>[4x]PPYTVVYFPVRGRCAALRMLLADQGQSWKEEVVTVETWQEGSLKASCLYGQLPKFQDGDLTLYQSNTILRHLGRTLGLYGKDQQEAALVDMVNDGVED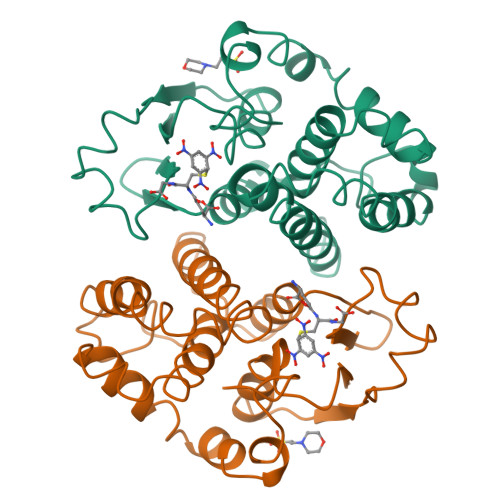LRCKYISLIYTNYEAGKDDYVKALPGQLKPFETLLSQNQGGKTFIVGDQISFADYNLLDLLLIHEVLAPGCLDAFPLLSAYVGRLSARPKLKAFLASPEYVNLPINGNGKQ> MNKPLTPSTYIRNLNVGILRKLSDFIDPQEGWKKLAVAIKKPSGDDRYNQFHIRRFEALLQTGLSPTCELLFDWGT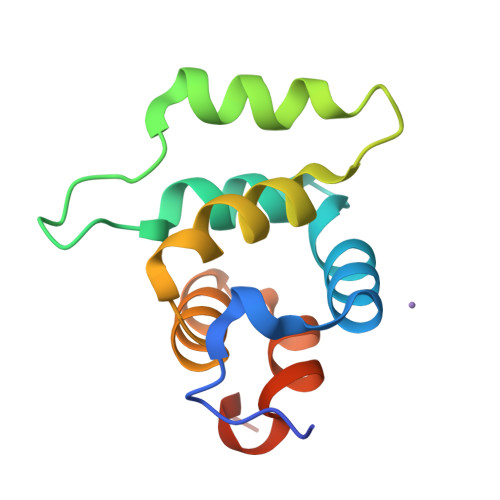TNCTVGDLVDLLVQIELFAPATLLLPDAVPQTVKSLP>[2x]MRGSHHHHHHGIPEFVNALVSHLLVVEPEKLYAMPDPAGPDGHLPAVATLCDLFDREIVVTISWAKS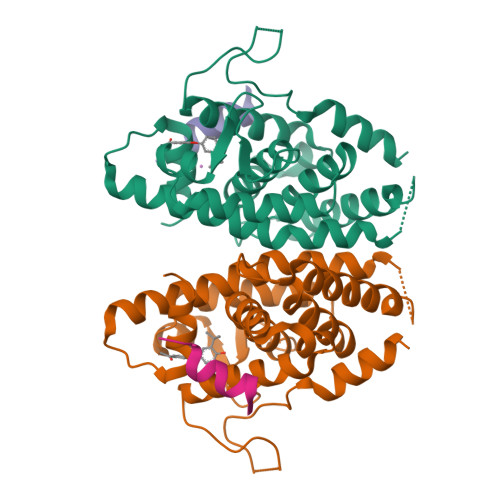IPGFSSLSLSDQMSVLQSVWMEVLVLGVAQRSLPLQDELAFAEDLVLDEEGARAAGLGELGAALLQLVRRLQALRLEREEYVLLKALALANSDSVHIEDAEAVEQLREALHEALLEYEAGRAGPGGGAERRRAGRLLLTLPLLRQTAGKVLAHFYGVKLEGKVPMHKLFLEMLEAMMD;>RPASELLKYLTT[2x]> MGSILTRWLLIPPVNARLIGRYRDYRRHGASAFSATLGCFWMILAWIFIPLEHPRWQRIRAEHKNLYPHINASRPRPLDPVRYLIQTCWLLIGASRKETPKPRRRAFSGLQNIRGRYHQWMNELPERVSHKTQHLDEKKELGHL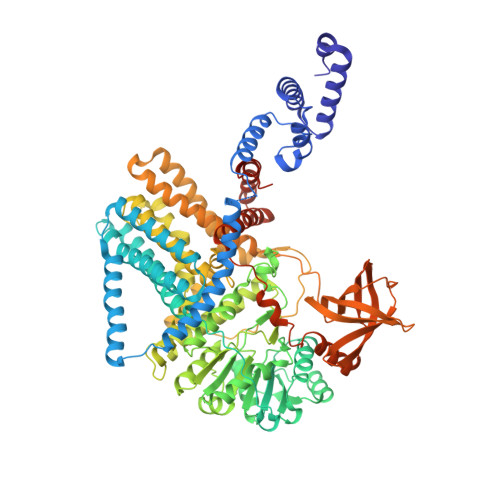SAGARRLILGIIVTFSLILALICVTQPFNPLAQFIFLMLLWGVALIVRRMPGRFSALMLIVLSLTVSCRYIWWRYTSTLNWDDPVSLVCGLILLFAETYAWIVLVLGYFQVVWPLNRQPVPLPKDMSLWPSVDIFVPTYNEDLNVVKNTIYASLGIDWPKDKLNIWILDDGGREEFRQFAQNVGVKYIARTTHEHAKAGNINNALKYAKGEFVSIFDCDHVPTRSFLQMTMGWFLKEKQLAMMQTPHHFFSPDPFERNLGRFRKTPNEGTLFYGLVQDGNDMWDATFFCGSCAVIRRKPLDEIGGIAVETVTEDAHTSLRLHRRGYTSAYMRIPQAAGLATESLSAHIGQRIRWARGMVQIFRLDNPLTGKGLKFAQRLCYVNAMFHFLSGIPRLIFLTAPLAFLLLHAYIIYAPALMIALFVLPHMIHASLTNSKIQGKYRHSFWSEIYETVLAWYIAPPTLVALINPHKGKFNVTAKGGLVEEEYVDWVISRPYIFLVLLNLVGVAVGIWRYFYGPPTEMLTVVVSMVWVFYNLIVLGGAVAVSVESKQVRRSHRVEMTMPAAIAREDGHLFSCTVQDFSDGGLGIKINGQAQILEGQKVNLLLKRGQQEYVFPTQVARVMGNEVGLKLMPLTTQQHIDFVQCTFARADTWALWQDSYPEDKPLESLLDILKLGFRGYRHLAEFAPSSVKGIFRVLTSLVSWVVSFIPRRPERSETAQPSDQALAQQHHHHHHLEHHHHHH>[2x]MALLEICCYSMECALTAQQNGADRVELCAAPKEGGLTPSLGVLKSVRQRVTIPVHPIIRPRG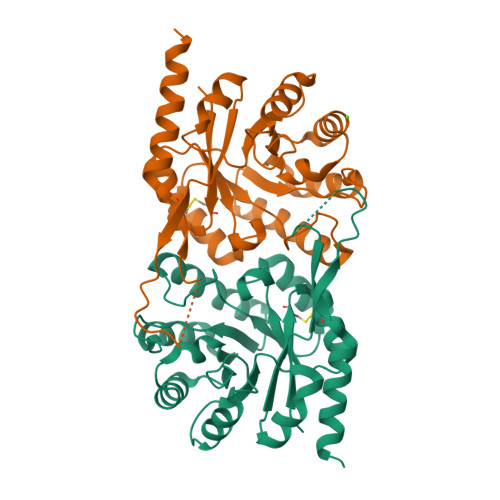GDFCYSDGEFAAILEDVRTVRELGFPGLVTGVLDVDGNVDMPRMEKIMAAAGPLAVTFHRAFDMCANPLYTLNNLAELGIARVLTSGQKSDALQGLSKIMELIAHRDAPIIMAGAGVRAENLHHFLDAGVLEVHSSAGAWQASPMRYRNQGLSMSSDEHADEYSRYIVDGAAVAEMKGIIERHQAKLEHHHHHH>[2x]MLSYRHSFHAGNHADVLKHT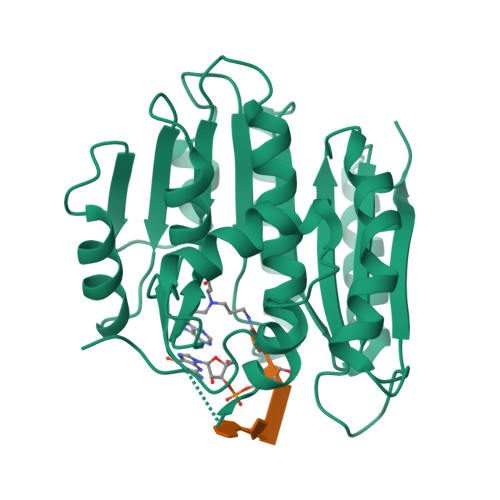VQSLIIESLKEKDKPFLYLDTHAGAGRYQLGSEHAERTGEYLEGIARIWQQDDLPAELEAYINVVKHFNRSGQLRYYPGSPLIARQLLREQDSLQLTELHPSDYPLLRSEFQKDSRARVEKADGFQQLKAKLPPVSRRGLILIDPPYEMKTDYQAVVSGIAEGYKRFATGTYALWYPVVLRQQIKRMIHDLEATGIRKILQIELAVLPDSDRRGMTASGMIVINPPWKLEQQMNNVLPWLHSKLVPAGTGHATVSWIVPE> NDPESALNRAVGRVADTVASGPVNTEQIPALTAVETGHTSQVVPSDTMQTRHVINYHTRSESSIENFMGRAACVYIAQYATEKVNDELDRYTNWEITTRQVAQLRRKLEMFTYMRFDLEITFVITSSQRTSTTYASDSPPLTHQVMYVPPGGPIPKSYEDFAWQTSTNPSVFWTEGNAPPRMSIPFMSVGNAYCNFYDGWSHFSQSGVYGYTTLNNMGHLYFRHVNKSTAYPVNSVARVYFKPKHVKAWVPRAPRLCPYLKARNVNFNVQGVTESRNKITLDRSTHNPLANT;> SPTVEECGYSDRVRSITLGNSTITTQECANVVVGYGVWPTYLSDHEATAVDQPTQPDVATCRFYTLESVKWE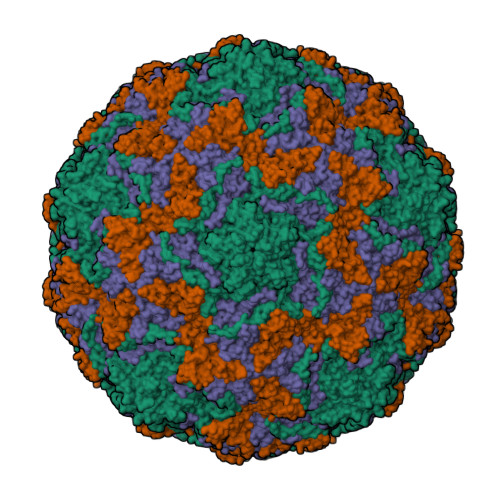SSSAGWWWKFPEALSDMGLFGQNMQYHYLGRTGYTIHVQCNASKFHQGCLLVVCVPEAEMGAATTDHAFNHTKLSNIGQAMEFSAKKSTDQTGPQTAVHNAGMGVAVGNLTIFPHQWINLRTNNSATIVMPYINSVPMDNMYRHYNFTLMVIPFAKLEHSPQASTYVPITVTVAPMCAEYNGLRLAGHQ;> GLPTMNTPGSTQFLTSDDFQSPSAMPQFDVTPEIQIPGQVRNLMEIAEVDSVVPVNNTEGHVNSMEAYRIPVRPQTSSGEQVFGFQLQPGHDSVLKHTLLGEILNYYANWSGSMKLTFMYCGAAMATGKFLIAYSPPGAGVPGSRRDAMLGTHVIWDVGLQSSCVLCVPWISQTNYRYVTSDAYTDAGYITCWYQTSIVTPPDIPTTSTILCFVSACNDFSVRLLRDTPFITQQALFQ;> XGAQVSTQKTGAHETGLNASGNSIIHYTNINYYKDSASNSLNRQDFTQDPSKFTEPVKDVMIKTLPALN>MRRMRLGTVLLVSPKTSFGRDLQRTYAGGLGTVCKDEDFLLPPLDLMRLAGVLREDADDIAIADEEVTGVVPSVEPGTTVICHVSLPSLLEDAERLATFRAQGARCYAYTSIRSPAQWRTLFERGGCEGVLLPESISFARAALAGDHTVPGLVTPDSLLDPRHHQPAFGDLAAEPLPARDLVDHTPYMFPPIARTGITSINGSFGCPYPCRFYCPYPLSEGRKIRTYPVERIVAEFRQCAELGITAAVFRDPVFSFHRDRTLELCQALKAADTGVPWWCETRIDRLDEEVVAALVDAGCVGVEVGVESGDPDMQATAVRKRLNLDTVRKFHAVARKAGLKLVFLFLIGLPRETRMSIRRTFDFILELGLADTEFNLSVITPYPGTELHQIAVDKGWIDGSQNAFTSHNAVMHTDELSIGDLERASRFVDELHAVCKAGPAERAEFQARVH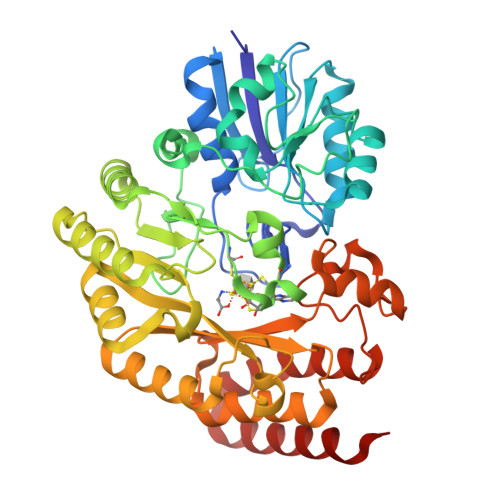AWSTGDA[2x]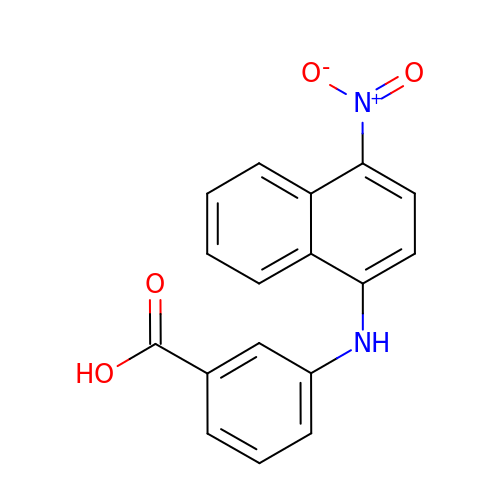3-[(4-nitronaphthalen-1-yl)amino]benzoic acid | C17 H12 N2 O4 | ZLIDMWNTWSBTSM-UHFFFAOYSA-N>GPMADPWQECMDYAVTLARQAGEVVCEAIKNEMNVMLKSSPVDLVTATDQKVEKMLISSIKEKYPSHSFIGEESVAAGEKSILTDNPTWIIDPIDGTTNFVHRFPFVAVSIGFAVNKKIEFGVVYSCVEGKMYTARKGKGAFCNGQKLQVSQQEDITKSLLVTE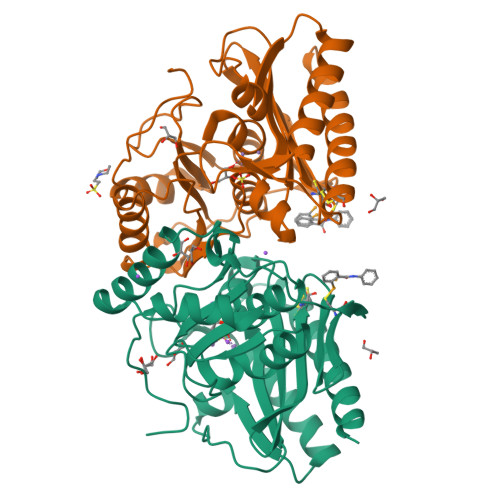LGSSRTPETVRMVLSNMEKLFCIPVHGIRSVGTAAVNMCLVATGGADAYYEMGIHCWDVAGAGIIVTEAGGVLMDVTGGPFDLMSRRVIAANNRILAERIAKEIQVIPLQRDDED[2x]>[2x]AAQCFLIDKNFVNKAVESANLTKDDVVLEIGLGKGILTEELAKNAKKVYVIEIDKSLEPYANKLKELYNNIEIIWGDALKVDLNKLDFNKVVANLPYQISSPITFKLIKRGFDLAVLMYQYEFAKRMVAKEGTKDYGRLSVAVQSRADVEIVAKVPPSAFYPKPKVYSAI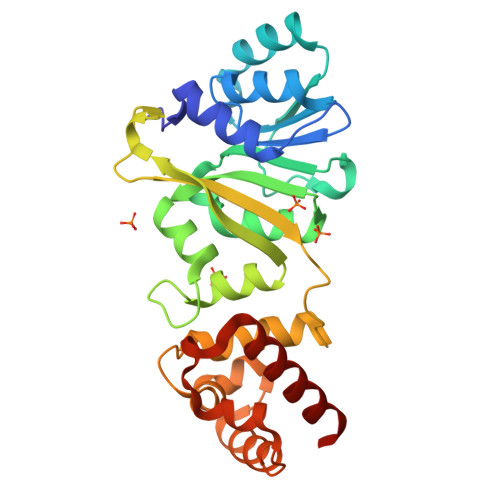VKIKPNKGKYHIENENFFDDFLRAIFQHRNKSVRKALIDSSKELNYNKDEMKKILEDFLNTNSEIKNLINEKVFKLSVKDIVNLSNEFYRFLQNR> GPLGSNSFVGLRVVAKWSSNGYFYSGKITRDVGAGKYKLLFDDGYECD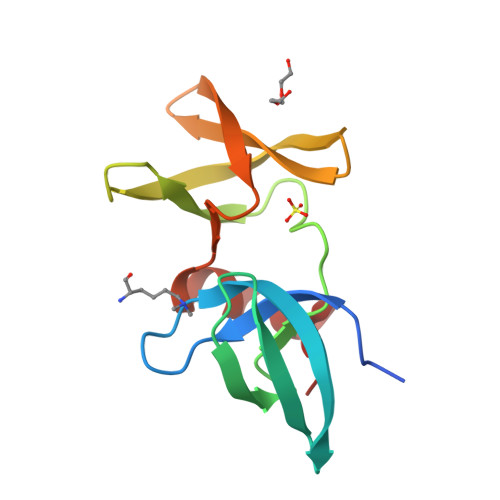VLGKDILLCDPIPLDTEVTALSEDEYFSAGVVKGHRKESGELYYSIEKEGQRKWYKRMAVILSLEQGNRLREQYGLG;> TSRHKKLMFKT>MKENEILRRELDRMRVPPLIVGTVVDKVGERKVVVKSSTGPSFLVNVSHFVNPDDLAPGKRVCLNQQTLTVVDVLPELEHHHHHH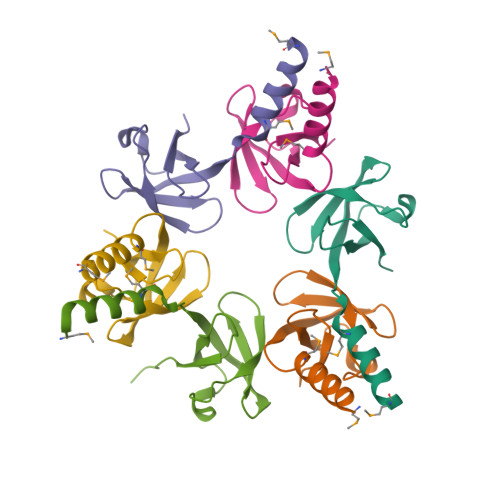[12x]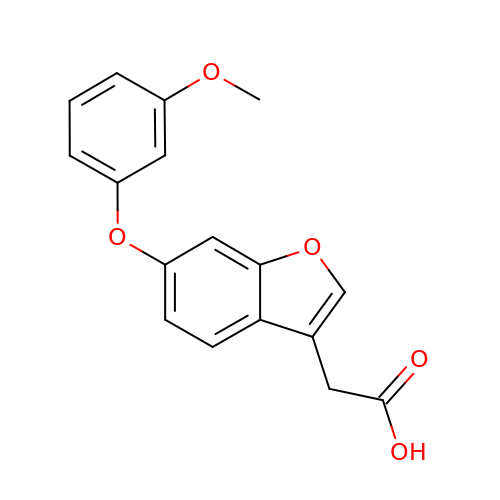[6-(3-methoxyphenoxy)-1-benzofuran-3-yl]acetic acid | C17 H14 O5 | UOSYUXUYPKFRGA-UHFFFAOYSA-N In this work, we exhaustively probe the ability of all 36 immobile HJ sequences to form DNA crystals in two different designed systems. Three separate self-assembling DNA crystal systems are described in this report: the “4 × 5” and “4 × 6” designs (collectively referred to as the 4 × N systems), and a third construct with a “scrambled” sequence variant of the 4 × 6 lattices. Self-assembly was mediated by three constituent oligonucleotides: (S1) containing four sequence repeats of either 5 or 6 bases; (S2) composed of 21 bases containing complementary regions to both (S1); and (S3) which forms the second junction crossover. The HJ serves as the fundamental component at the core of each unit, and the ultimate assembly of the full lattice is facilitated by the complementary 2-base sticky ends that tail each duplex.

The layered motif provided a well-defined scaffold at 3.1 Å resolution, but the aperiodicity of the cavities and corresponding volumes would be inadequate for scaffolding guest materials. We hypothesized that it might be possible to introduce other unique immobile sequences that could provide slight perturbations in the junction angle, to potentially reduce the strain in the original system and yield a “relaxed,” periodic lattice. The 4 × 5 system robustly crystallized with 75% of the junctions, and we obtained crystals in all but 9 of 36 sequences. Although the cell parameters between the two symmetries were virtually indistinguishable, the differences between the periodicity of the lattices is dramatic, with vastly different cavity sizes. While the highest resolution achieved for the J1 system was 3.1 Å, in roughly half of the crystals measured the resolutions were 3.05 Å or better, and as high as 2.9 Å (J6) and 2.75 Å (J19), for the P32 and P3221 symmetries, respectively. Of the resulting structures, 18 exhibited P32 symmetry with average cell dimensions a = b = 68.85 Å c = 60.09 Å, with only nine retaining the original P3221 symmetry with average cell edges a = b = 68.17 Å c = 60.60 Å. We show that J1 (or any other junction) should not be considered a privileged option for designing self-assembled lattices. However, in the majority of the crystal structures reported here, the cacodylate anion indeed fits best into the electron density map of our X-ray structures, due to the presence of sodium cacodylate in the crystallization solution.

> GAGCAGACCTG;> ACGACACTCA;> CACGT;> TCTGAGTGTGGTCTGC>GHMSETYDFLFKFLVIGNAGTGKSCLLHQFIEKKFKDDSNHTIGVEFGSKIINVGGKYVKLQIWDTAGQERFRSVTRSYYRGAAGALLVYDITSRETYNALTNWLTDARMLASQNIVIILCGNKKDLDADREVTFLEASRFAQENELMF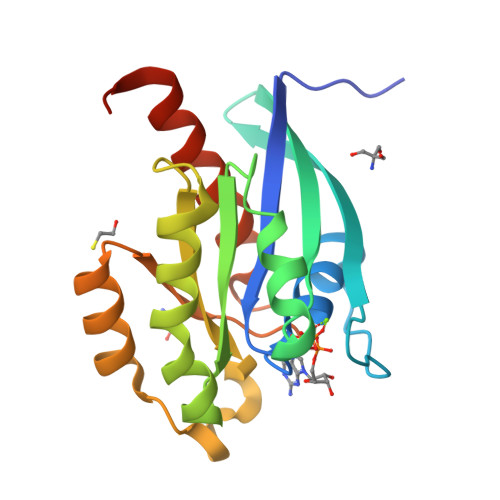LETSALTGENVEEAFVQCARKILNKIESGELDPERMG[4x]>[2x]MRSRRVDVMDVMNRLILAMDLMNRDDALRVTGEVREYIDTVKIGYPLVLS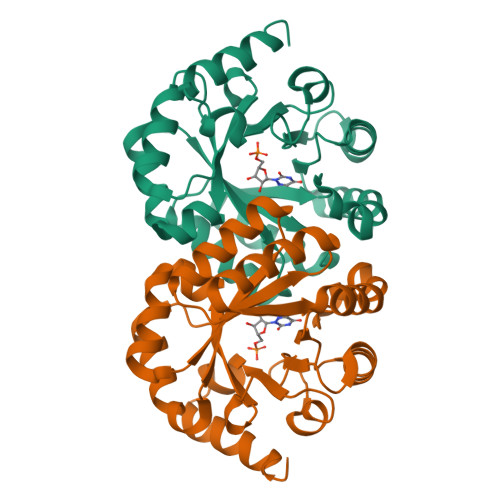EGMDIIAEFRKRFGCRIIADFKVADIPETNEKICRATFKAGADAIIVHGFPGADSVRACLNVAEEMGREVFLLTEMGHPGAEMFIQGAADEIARMGVDLGVKNYVGPSTRPERLSRLREIIGQDSFLISPGVGAQGGDPGETLRFADAIIVGRSIYLADNPAAAAAGIIESIKDLLNP>[2x]MSFVITNPEALTVAATEVRRIRDRAIQSDAQVAPMTTAVRPPAADLVSEKAATFLVEYARKYRQTIAAAAVVLEEFAHALTTGADKYATAEADNIKTFS;>MAFEAYPPEVNSANIYAGPGPDSMLAAARAWR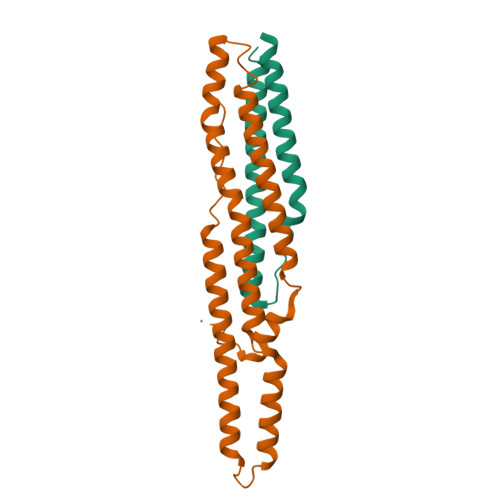SLDVEMTAVQRSFNRTLLSLMDAWAGPVVMQLMEAAKPFVRWLTDLCVQLSEVERQIHEIVRAYEWAHHDMVPLAQIYNNRAERQILIDNNALGQFTAQIADLDQEYDDFWDEDGEVMRDYRLRVSDALSKLTPWKAPPPIAHSTVLVAPVSPSTASSRTDTLVPR[2x]> ATTLKEAADGAGRDFGFALDPNRLSEAQYKAIADSEFNLVVAENAMKWDATEPSQNSFSFGAGDRVASYAADTGKELYGHTLVWHSQLPDWAKNLNGSAFESAMVNHVTKVADHFEGKVASWDVVNEAFADGGGRRQDSAFQQKLGNGYIETAFRAARAADPTAKLCINDYNVEGINAKSNSLYDLVKDFKARGVPLDCVGFQSHLIVGQVPGDFRQNLQRFADLGVDVRITELDIRMRTPSDATKLATQAADYKKVVQACMQVTRCQ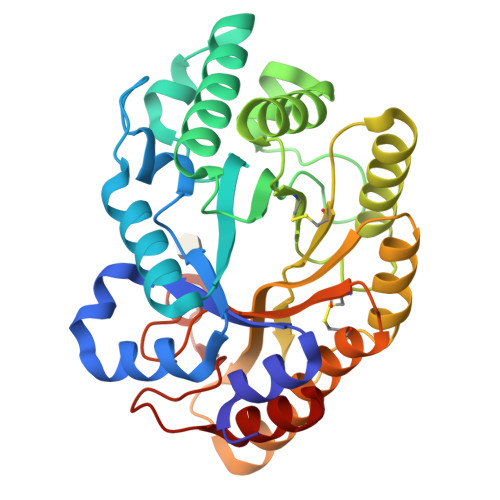GVTVWGITDKYSWVPDVFPGEGAALVWDASYAKKPAYAAVMEAFGAS> MESIEQQLTELRTTLRHHEYLYHVMDAPEIPDAEYDRLMRELRELETKHPELITPDSPTQRVGAAPLAAFSQIRHEVPMLSLDNVFDEESFLAFNKRVQDRLKNNEKVTWCCELKLDGLAVSILYENGVLVSAATRGDGTTGEDITSNVRTIRAIPLKLHGENIPARLEVRGEVFLPQAGFEKINEDARRTGGKVFANPRNAAAGSLRQLDPRITAKRPLTFFCYGVGVLEGGELPDTHLGRLLQFKKWGLPVSDRVTLCESAEEVLAFYHKVEEDRPTLGFDIDGVVIKVNSLAQQEQLGFVARAPRWA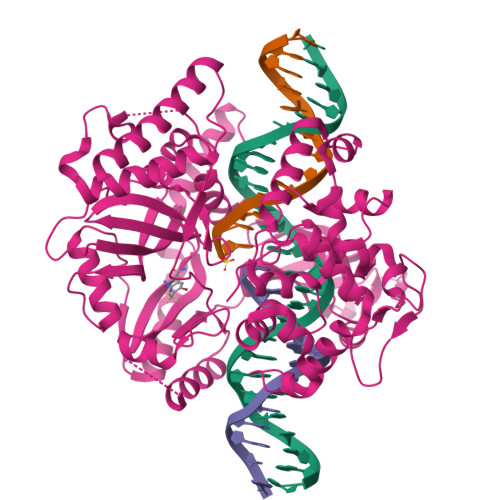VAFKFPAQEQMTFVRDVEFQVGRTGAITPVARLEPVHVAGVLVSNATLHNADEIERLGLRIGDKVVIRRAGDVIPQVVNVVLSERPEDTREVVFPTHCPVCGSDVERVEGEAVARCTGGLICGAQRKESLKHFVSRRAMDVDGMGDKIIDQLVEKEYVHTPADLFKLTAGKLTGLERMGPKSAQNVVNALEKAKETTFARFLYALGIREVGEATAAGLAAYFGTLEALEAASIEELQKVPDVGIVVASHVHNFFAEESNRNVISELLAEGVHWPAP> MAHHHHHHMSAQVMLEEMARKYAINAVKADKEG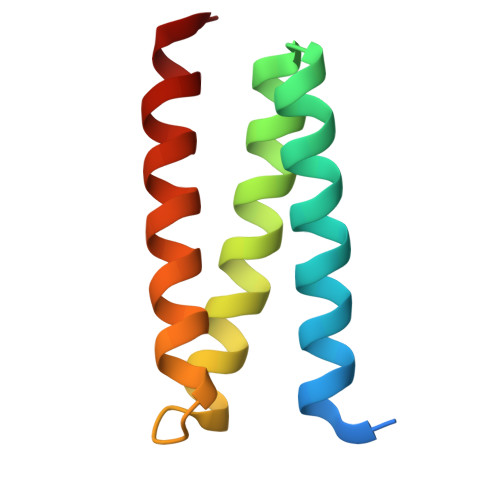NAEEAITNYKKAIEVLAQLVSLYRDGSTAAIYEQMINEYKRRIEVLKELI>[2x]PVSMTYLYNKYSFKLILAEYIRHRNTIS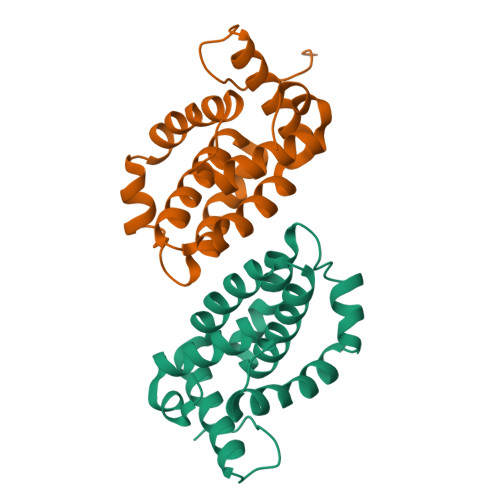GNIYSALMTLDDLAIKQYGDIDLLFNEKLKVDSDSGLFDFVNFVKDMICCDSRIVVALSSLVSKHWELTNKKYRCMALAEHISDSIPISELSRLRYNLCKYLRGHTESIEDEFDYFED> SHNMSLPQWCPPHSTLKRNPTTGEDVYCICKRPDYGELMVGCDGCDDWFHFTCL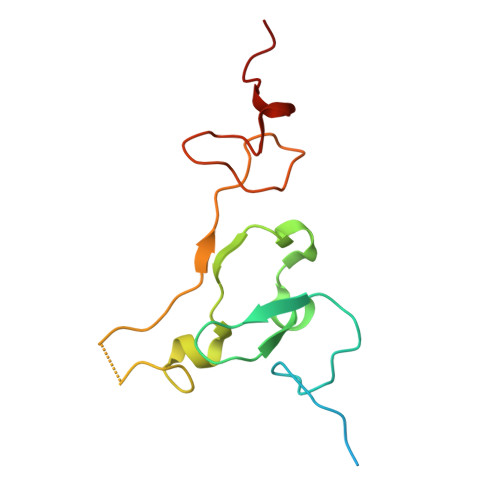HIPEQFKDLVFSFYCPYCQAGITGKNKNGEGSLPKTLWKRKCRISDCYKPCLQDSKYCSEEHGREFVND>MTEDRLSAEDKKFLEVERALKEAALNPLRHATEELFGDFLKMENITEICYNGNKVVWVLKNNGEWQPFDVRDRK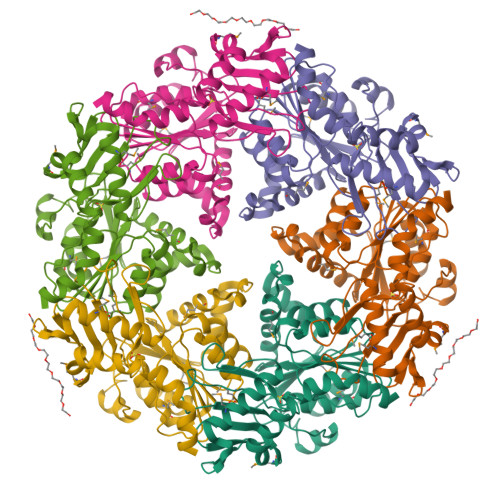AFSLSRLMHFARCCASFKKKTIDNYENPILSSNLANGERVQIVLSPVTVNDETISISIRIPSKTTYPHSFFEEQGFYNLLDNKEQAISAIKDGIAIGKNVIVCGGTGSGKTTYIKSIMEFIPKEERIISIEDTEEIVFKHHKNYTQLFFGGNITSADCLKSCLRMRPDRIILGELRSSEAYDFYNVLCSGHKGTLTTLHAGSSEEAFIRLANMSSSNSAARNIKFESLIEGFKDLIDMIVHINHHKQCDEFYIKHR[2x]We reasoned that to enable systematic design of binders to convex protein target sites it would be necessary to generate scaffold sets with overall concave shapes. We focused on 5 helix bundle scaffolds with three helices forming the concave interface and two helices providing structural support. The selected 7476 scaffolds, which we refer to as 5HCS (5 helix concave scaffolds) throughout the remainder of the text, have a wide range of curvatures. Our method for computationally designing small but concave proteins to bind to convex protein target sites expands the space of the protein surfaces that can be targeted by de novo protein design.

Because of the therapeutic importance of the target, and receptor extracellular Ig domains more generally, we next sought to evaluate the generality of our approach by designing 5HCS based binders to CTLA-4. CTLA-4 plays an important role in peripheral tolerance and the prevention of autoimmune disease by inhibition of T cell activation. Deep sequencing of a site saturation mutagenesis library of the most enriched binder, 5HCS_CTLA4_0, showed that the designed core and interfacial residues of the binder were highly conserved, suggesting the design folds and binds target as in the computational model. We determined co-crystal structures of 5HCS_CTLA4_1 with CTLA-4 and unbound crystal structures of 5HCS_CTLA4_2. The unbound crystal structure of 5HCS_CTLA4_2 aligns with the structure of binder in 5HCS_CTLA4_1 bound structure well with a rmsd. of 0.416 Å. The circular dichroism spectra indicates a helical structure with peaks at 208 nm and 222 nm consistent with the design model and was unchanged by heating to 95 °C, indicating high thermal stability.

> SNNLEEEVQKLLYELSEIWHQHDHEASREALHRVLEVLKQLLEHNNLEQAVELISIAVHVAVRVNNEHVIRELHHLLRRLLKQVKEHNNNKLYIAVMSVIMQLERT7-(pyridin-2-ylmethyl)quinolin-8-ol | C15 H12 N2 O | 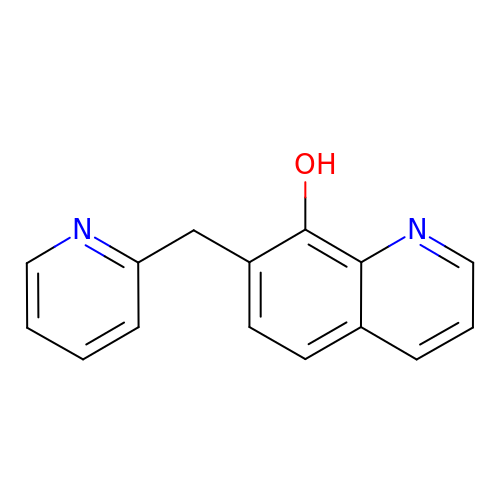WLWQZKQFQNNCAP-UHFFFAOYSA-N>[4x]SNAMSQFMNLEGKVALVTGASRGIGKAIAELLAERGAKVIGTATSESGAQAISDYLGDNGKGMALNVTNPESIEAVLKAITDEFGGVDILVNNAGITRDNLLMRMKEEEWSDIMETNLTSIFRLSKAVLRGMMKKRQGRIINVGSVVGTMGNAGQANFAAAKAGVIGFTKSMAREVASRGVTVNTVAPGFIETDMTKALNDEQRTATL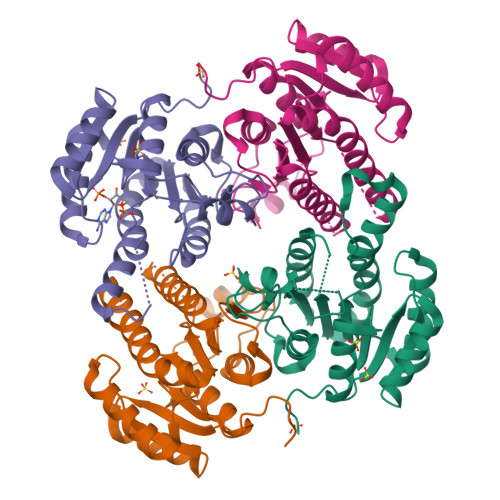AQVPAGRLGDPREIASAVAFLASPEAAYITGETLHVNGGMYMI>MAS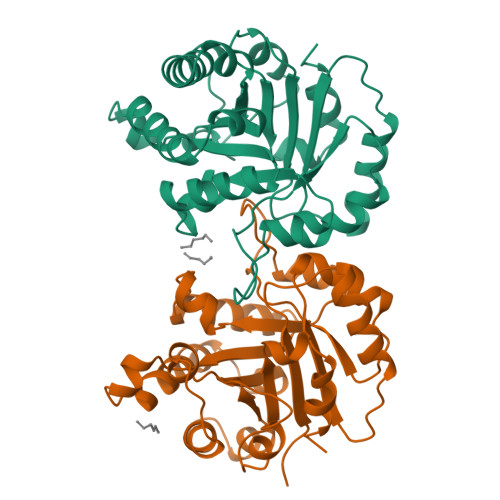KPQPIAAANWKCNGSESLLVPLIETLNAATFDHDVQCVVAPTFLHIPMTKARLTNPKFQIAAQNAITRSGAFTGEVSLQILKDYGISWVVLGHSERRLYYGETNEIVAEKVAQACAAGFHVIVCVGETNEEREAGRTAAVVLTQLAAVAQKLSKEAWSRVVIAYEPVWAIGTGKVATPQQAQEVHELLRRWVRSKLGTDIAAQLRILYGGSVTAKNARTLYQMRDINGFLVGGASLKPEFVEIIEATK[2x]>[2x]MTIKWIDWVKQIQSIAQAGLTYSKDVYDIERFQQLRDISISMMSHYTKTDWEVVEKLFASETGYQTPKVDIRAVVFQNEKLLFVKEKSDGKWALPGGWADVGYTPTEVAAKEVFEETGYEVDHFKLLAIFDKEKHQPSPSATHVYKIFIGCEIIGGEKKTSIETEEVEFFGENELPNLSIARNTEDQIKEMFAYMKDPQKEKLID

The two recently opened beamlines for macromolecular crystallography at NSLS-II have launched the microcrystallography field into new territory, with flux densities up to two orders of magnitude brighter than those previously available. In this study, we highlight the capabilities of the AMX and FMX beamlines at NSLS-II by describing structure determination from single crystal vector data collection and two methods for multicrystal data collection. The advent of next generation synchrotron beamlines has necessitated the development of new strategies to fully benefit from the increased beam intensity and smaller beam sizes while minimizing radiation damage. The high dose rates, in conjunction with the newly developed ultrafast raster scanning goniometer brings formerly time-consuming serial crystallography measurements into the minutes range. These new opportunities mean that inhomogeneous large crystals can now deliver high quality data collected from their best volume, and crystals as small as 5 to 10 µm can deliver one or more complete datasets.

B. cereus CDP-Chase is a member of the Nudix hydrolase superfamily, which are a family of enzymes that hydrolyze nucleoside diphosphates linked to some other moiety, x. It is a bifunctional enzyme that can hydrolyze CDP-choline with the typical nudix reaction in addition to a non-nudix exonuclease reaction on RNA. Here, we have described the determination of two CDP-Chase structures cocrystallized with ADP-ribose. For the sake of comparison between the single and multicrystal data collection methods, we collected data of CDP-Chase on both a single crystal and using the raster data collection. A total of 119 partial datasets were collected and processed using the Python scripted workflow described previously relying on DOZOR, XDS, POINTLESS, and AIMLESS. The dataset was refined to a final resolution of 2.0 Å using iterative rounds of refinement with REFMAC5 and manual rebuilding in Coot. As might be expected, the Rmerge is much higher in the multicrystal dataset compared with the single crystal (35.7% compared with 13.6%). Since Rmerge fails to take into account higher redundancy, both the Rpim and CC1/2 were considered and found to be reasonable (13.7% and 94.1%, respectively), emphasizing the need to look at multiple measures to assess data quality, particularly in the case of datasets derived from multiple crystals. The level of detail observed in both electron density maps is comparable, and the RMSD between the refined structures is 0.11 Å. Despite the less favorable statistics for the multicrystal dataset in both the collection and refinement stages, the similarities of the two structures highlight the reliability and applicability of this method when larger crystals are not available, even for ligand or small molecule bound structures.BbvCI, a Type IIT restriction endonuclease, recognizes and cleaves the seven base pair sequence 5′-CCTCAGC-3′, generating 3-base, 5′-overhangs. BbvCI is composed of two protein subunits, each containing one catalytic site. Either site can be inactivated by mutation resulting in enzyme variants that nick DNA in a strand-specific manner. Earlier mutagenesis of these residues confirmed their catalytic nature and demonstrated that the site in the R1 subunit cleaves the bottom strand of the target site, while the site in the R2 subunit cleaves the top strand.

Purified samples of wild-type BbvCI, containing a 1:1 ratio of R1 and R2 subunits yielded crystals under acidic conditions (pH 4.5) in the presence of an excess of duplex DNA oligo containing the target site, and 2 mM calcium chloride. The crystals of the native protein diffracted strongly to 2.1 Å resolution, and belong to space group C222, with three subunits (1 +1/2 dimers) in the asymmetric unit. We initially calculated MIR phases, built an initial structure, and conducted refinements using datasets corresponding to the latter (heavy-atom) space group, and then subsequently determined the final, higher resolution structure of the native (non-derivatized) protein in the original C222 space group via molecular replacement and phase extension. The resulting electron density maps clearly corresponded to two full-length protein chains, but no density corresponding to DNA was present. In contrast, modeling the electron density as a homodimer comprising two copies of the R2 subunit resulted in satisfactory values for Rwork and Rfree (0.189/0.249, respectively), excellent correlation of the model to experimental electron density, and significantly improved geometric quality. The dimensions of the homodimer are ∼100 Å × 50 Å × 50 Å. The molecule is saddle-shaped due to deep concave surfaces at the dimer interface, and there is no obvious region of contiguous positive surface charge that might accommodate a DNA duplex of seven or more base pairs. Within each R2 subunit, the PD-(D/E)XK catalytic site occurs in its customary position, at the termini of adjacent beta-strands in the core domain. However, the two sites in the protein dimer are located ∼45 Å apart from one another–too far away from each other to catalyze double-strand cleavage reactions producing a 3-base overhang.

>MFNQFNPLVYTHGGKLERKSKKDKTASKVFEEFGVMEAYNCWKEASLCIQQRDKDSVLKLVAALNTYKDAVEPIFDSRLNSAQEVLQPSILEEFFEYLFSRIDSIVGVNIPIRHPAKGYLSLSFNPHNIETLIQSPEYTVRAKDHDFIIGGSAKLTIQGHGGEGETTNIVVPAVAIECKRYLERNMLDECAGTAERLKRATPYCLYFVVAEYLKLDDGAPELTEIDEIYILRHQRNSERNKPGFKPNPIDGELIWDLYQEVMNHLGKIWWDPNSALQRGKVFNRP[3x]>[2x]SMDEPDMISVFIGTWNMGSVPPPKNVTSWFTSKGLGK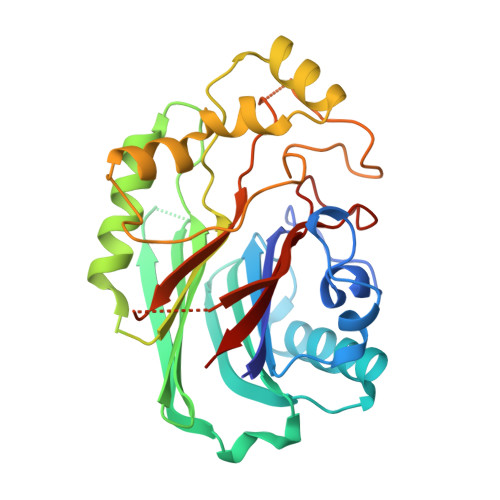TLDEVTVTIPHDIYVFGTQENSVGDREWLDLLRGGLKELTDLDYRPIAMQSLWNIKVAVLVKPEHENRISHVSTSSVKTGIANTLGNKGAVGVSFMFNGTSFGFVNCHLTSGNEKTARRNQNYLDILRLLSLGDRQLNAFDISLRFTHLFWFGDLNYRLDMDIQEILNYISRKEFEPLLRVDQLNLEREKHKVFLRFSEEEISFPPTYRYERGSRDTYAWHKQKPTGVRTNVPSWCDRILWKSYPETHIICNSYGCTDDIVTSDHSPVFGTFEVGVTSQ> MSLGAKPF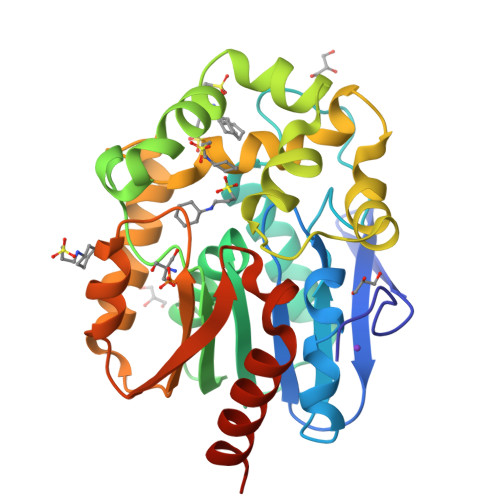GEKKFIEIKGRRMAYIDEGTGDPILFQHGNPTSSYLWRNIMPHCAGLGRLIACDLIGMGDSDKLDPSGPERYAYAEHRDYLDALWEALDLGDRVVLVVHDWGSALGFDWARRHRERVQGIAYMEAIAMPIEWADFPEQDRDLFQAFRSQAGEELVLQDNVFVEQVLPGLILRPLSEAEMAAYREPFLAAGEARRPTLSWPRQIPIAGTPADVVAIARDYAGWLSESPIPKLFINAEPGALTTGRMRDFCRTWPNQTEITVAGAFFIQEDSPDEIGAAIAAFVRRLRPAHHHHHH> SNAPLVKRLREQPQNILT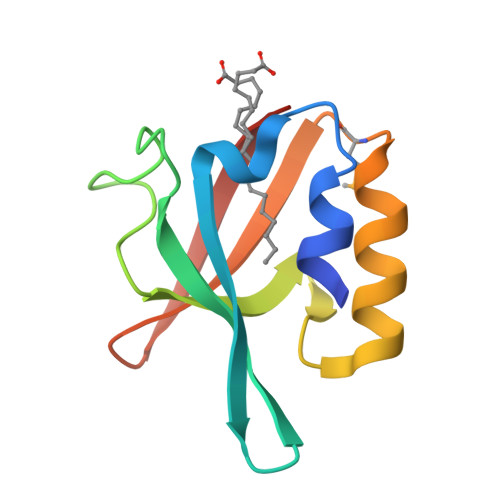YLSISPVLSGDKLLGYRLNPGKDASLFRQSGLQANDLAIALNGIDLRDQEQAQQALQNLADMTEITLTVEREGQRHDIAFALGDE>MHHHHHHPMEPEIKIVNVVVSTKIGDNIDLEEVAMILENAEYEPEQFPGLVCRLSVPKVALL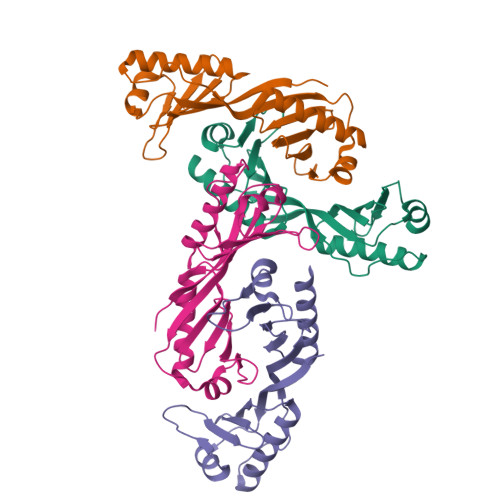IFRSGKVNCTGAKSKEEAEIAIKKIIKELKDAGIDVIENPEIKIQNMVATADLGIEPNLDDIALMVEGTEYEPEQFPGLVYRLDDPKVVVLIFGSGKVVITGLKSEEDAKRALKKILDTIKEVQEL[4x]> GVNLEAFSQAIS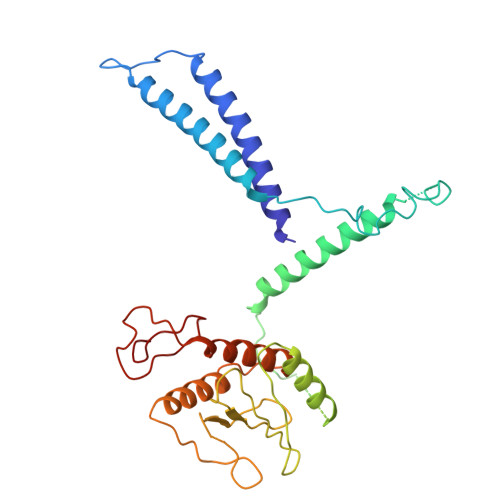AIQALRSSVSRVFDCLKDGMRNKETLEGREKAFIANFQDNLHSVNRDLNELERLSNLVGKPSENHPLHNSGLLSLDPVQDKTPLYSQLLQAYKWSNKLQYHAGLASGLLNQQSLKRSANQMGVSAKRRPKAQPTTLVLPPQYVDDVISRIDRMFPEMSIHLSRPNGTSAMLLVTLGKVLKVIVVMRSLFIDRTIVKGYNESVYTEDGKLDIWSKSSYQVFQKVTDHATTALLHYQLPQMPDVVVRSFMTWLRSYIKLFQAPCQRCGKFLQDGLPPTWRDFRTLEA> MVAYDNKNNEGFSPNLPEMTGTTIMAVKYADGILIGADCRTSMGTYVSSRFTDKLTKISDNIYCCRSGSAADTQAITQYITELVQRSSFIDKEIPSVKKAAMAAKDIIYRYPNMLAGLIIAGYDTKPRIFNISLGGTMTEAEWQIGGSGSAYIYGLC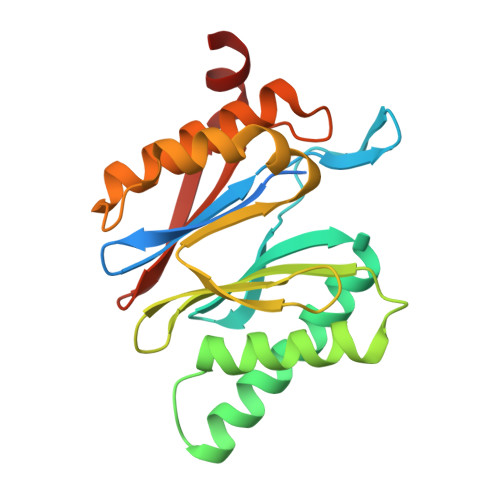DTTFKPNMNLEEALEFVKLAVTCAIKRDNASGGCIRMASITREGVQRFFYSGDKILNST IadA is a binuclear metalloenzyme and a member of the amidohydrolase superfamily. This enzyme catalyzes the hydrolytic cleavage of β-aspartyl dipeptides. In the present study, we determined the crystal structures of IadA from Colwellia psychrerythraea strain 34H (CpsIadA) in its ligand-free form and that in complex with β-isoaspartyl lysine, and subsequently characterized its enzymatic properties. The CpsIadA monomer structure contains ten α-helices and eighteen β-strands, and the overall structure is divided into two distinct domains (a β-sandwich domain and a catalytic domain).

Two Zn ions are located in the central cavity of the αβ-barrel structure. Although no exogenous metal ions were added to the CpsIadA protein solution during purification or crystallization, two strong electron densities were identified in the Fo-Fc map. We performed an X-ray fluorescence scan using the crystal to determine the identity of the metal. The result showed that a strong fluorescence signal was detected near the zinc K absorption edge and that the emission peaks from this scan were unambiguously characteristic for zinc. The CpsIadA active site contains two Zn ions (ZN1 and ZN2) with the ions being separated by 3.2 Å in distance. ZN2 interacts with the OE1 atom of Glu166, the ND1 atom of His205, and the NE2 atom of His234. Notably, Glu166 directly interacts with the Zn ions in the CpsIadA structure. The antiparallel β14 and β15 strands are located near the metal binding site and appear to form the gate for substrate entry or product release because of the relatively high B-factors observed in this region. In the crystal structure of the ligand-free CpsIadA, this part of the β14 and β15 region (residues 297–312) was disordered. The final model of ligand-free CpsIadA had an Rwork and an Rfree of 16.3% and 20.1%, respectively.

>[2x]MNDSQTMLILLCNVNIYAPNPLGIKDVLIAGNKIAAIYDHGQGEITIPKQWPVKVINFDGAILTPGFIDSHAHITGGGGEAGFATQVPPVGLTEFTHAGVTTVVGLLGTDDTTRSTENLLSRVYGLREEGLSAYCWTGGYHFPLTTITGSAKSDIAFLEPVIGIGEFAISDHRSSQPTFEEVIRLASETHVAGLITGKAGVIHFHLGDGERRLELIERAIRETELPARVFNPTHVNRNKPLFEDSCKLLSKGCHIDLTAFPAGTAQPGWEACDAIEMAVERQLPLEQITLSSDGGGCLPCFDPQGELQHMDFGRASTLGETLVATLNKGLSLETVLPMLTSNVANILRFKNKGQIAVGFDADLLVMNEKYEITDVMAQGVWHKQNNQTMIKGTFE> MAATAAEAVASGSGEPREEAGALGPAWDESQLRSYSFPTRPIPRLSQSDPRAEELIENEEPVVLTDTNLVYPALKWDLEYLQENIGNGDFSVYSASTHKFLYYDEKKMANFQNFKPRSNREEMKFHEFVEKLQDIQQRGGEERLYLQQTLNDTVGRKIVMDFLGFNWNWINKQQGKRGWGQLTSNLLLIGMEGNVTPAHYDEQQNFFAQIKGYKRCILFPPDQFECLYPYPVHHPCDRQSQVDFDNPDYERFPNFQNVVGYETVVGPG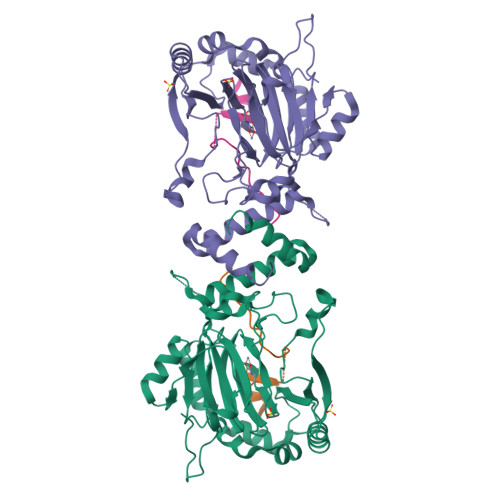DVLYIPMYWWHHIESLLNGGITITVNFWYKGAPTPKRIEYPLKAHQKVAIMRNIEKMLGEALGNPQEVGPLLNTMIKGRYN;> PSDLACRLLGQSMDESGLPQLTSYDCEVNAPIQGSRNLLQGEELLRALDQVN Recently, a fluorophore named 5-((Z)-4-((2-hydroxyethyl)(methyl)amino)benzylidene)-3-methyl-2-((E)-styryl)-3,5-dihydro-4H-imidazol-4-one (NBSI), emitting in red spectrum, and its cognate aptamer named Clivia were identified, exhibiting a large Stokes shift. The overall structure uses a monomeric, non-G-quadruplex compact coaxial architecture, with NBSI sandwiched at the core junction. The overall structure of the complex adopts a coaxial long helix fold and is stabilized by continuous stacking interactions from the bottom stem P1 to the apical stem P2 with the ligand NBSI intercalated in the zipped junction region at the interface of stems P1 and P2. Our structural investigation of the Clivia aptamer bound to NBSI or NBSI derivatives revealed that the Clivia aptamer adopts a non-G-quadruplex scaffold supporting a specific ligand-binding pocket, suggesting a new fluorescence activation mechanism.

Two additional reported derivatives of NBSI, designated NBSI565 (3) and NBSI618 (4), were generated by introducing a 4-OH or 4-CN group to the styryl moiety of NBSI571, respectively. NBSI565 had an excitation maximum at 490 nm and an emission maximum at 565 nm, while its binding affinity was Kd = 22 nM. Our 3D fluorescence spectra of free NBSI565 in buffer and Clivia-bound NBSI565 revealed that free NBSI565 in buffer exhibited two excitation wavelength peaks at 382 and 552 nm, whereas Clivia-bound NBSI565 displayed only one excitation wavelength peak at 491 nm. Structure determination of the Clivia–NBSI565 complex demonstrated a remarkable resemblance of the binding pocket architecture to that of NBSI571 and NBSI. NBSI565 was stacked in the binding pocket with the attached 4-OH group residing at the terminus of the binding pocket.

>[2x]GAAGAUUGUAAACAUGCCGAAAGGCAGACACUUCC>[5x]TPDCVTGKVEYTKYNDDDTFTVKVGDKEL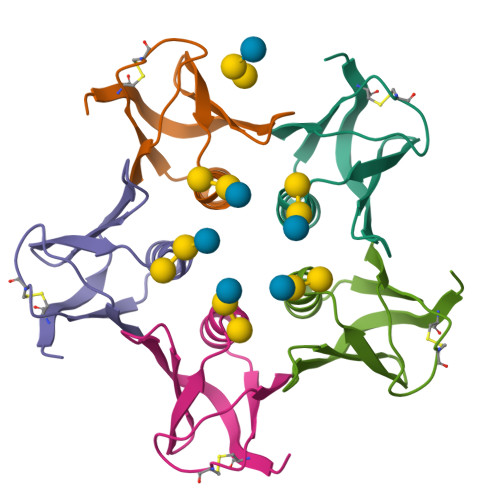FTNRWNLQSLLLSAQITGMTVTIKTNACHNGGTFSEVIFR>MHHHHHHAMAALRNRVFVIGVGMTKFEKPGARDIDYPDMAKEAGQRALADAGIKYSAIQQACVGYVYGDSTCGQRAIYHSLGLSGIPIINVNNNCSTGSTALFMGRQLIQGGLADCVLALGFEKMERGSLSSKYMDRTNPMDKHMEVMINRYGLAAVPAAPQMFGNAGREHMEKYGTKPEHFAKVAWKNHKHSTNNPYSQFQDEYSLEQVIDSRKVFEFLTLLQCCPTSDGAGAAVLASESFVRRNGLEKKAVEIVAQEMVTDLSTTFEENSCMKMVGYDMTRLAAERC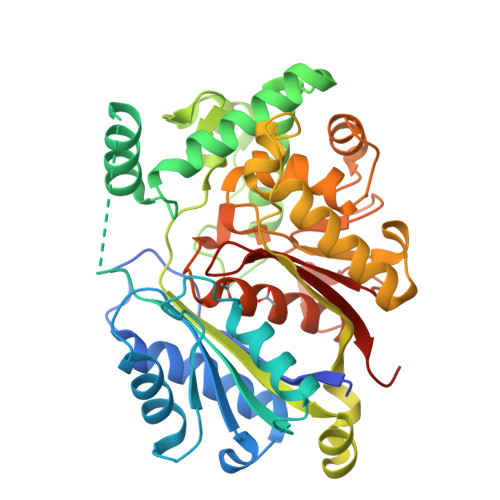YDTAGVKPSDVDVIELHDCFSANELITYEALGLCPEGKAGELIDRGDNTYGGKWVINPSGGLISKGHPLGATGLAQCAELCWQLRAEAGPRQVPGAKLALQHNIGLGGAVVVTLYKMGFPQETSS[2x]>GSHMHLTARGLTLDLSRPQVMGILNVTPDSFSDGGCHNNLDQALQHAQRMLSAGATLI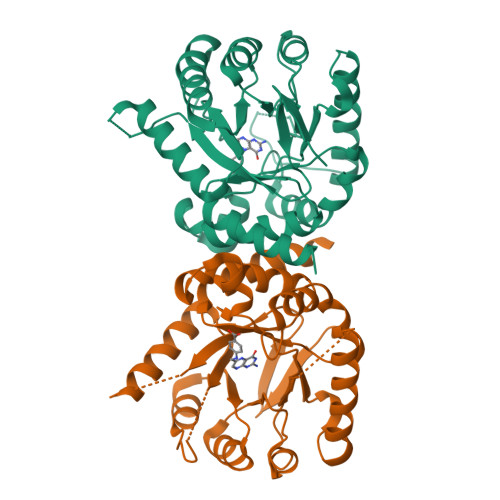DIGGESTRPGAAEVSEQEELDRVVPVVEALAQRFDVWLSVDTSKAAVITESAHAGAHLINDIRSLQEPGALEAAAKTGLPVCLMHMQGQPKNMQHSPYYDDLMTDINRFFQHHIERCVAAGIAKNKLLLDPGFGFGKNLAHNYQLLAHLSELHHFELPLLVGMSRKSMVGQLLNVPPQQRVIGSVACAVIAAMQGAQIIRVHDVKETVEAMCIVEATRSAKG[2x]> MSLAYKGYLIDLDGTIYKGKSRIPAGERFIERLQEKGIPYMLVTNNTTRTPE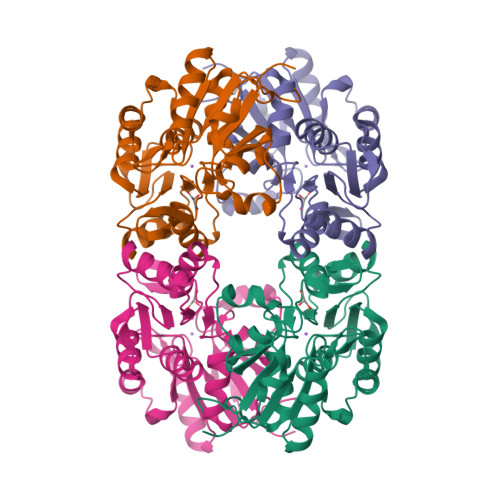SVQEMLRGFNVETPLETIYTATMATVDYMNDMNRGKTAYVIGEEGLKKAIADAGYVEDTKNPAYVVVGLDWNVTYDKLATATLAIQNGALFIGTNPDLNIPTERGLLPGAGSLNALLEAATRIKPVFIGKPNAIIMNKALEILNIPRNQAVMVGDNYLTDIMAGINNDIDTLLVTTGFTTVEEVPDLPIQPSYVLASLDEWTFNEGHHHHHH> MEDVEIKPRGYQLRLVDHLTKSNGIVYLPTGSGKTFVAILVLKRFSQDFDKPIESGGKRALFMCNTVELARQQAMAVRRCTNFKVGFYVGEQGVDDWTRGMWSDEIKKNQVLVGTAQVFLDMVTQTYVALSSLSVVIIDECHHGTGHHPFREFMRLFTIANQTKLPRVVGLTGVLIKGNEITNVATKLKELEITYRGNIITVSDTKEMENVMLYATKPTEVMVSFPHQEQVLTVTRLISAEIEKFYVSLDLMNIGVQPIRRSKSLQCLRDPSKKSFVKQLFNDFLYQMKEYGIYAASIAIISLIVEFDIKRRQAETLSVKLMHRTALTLCEKIRHLLVQKLQDMTYDDDDDNVNTEEVIMNFSTPKVQRFLMSLKVSFADKDPKDICCLVFVERRYTCKCIYGLLLNYIQSTPELRNVLTPQFMVGRNNISPDFESVLERKWQKSAIQQFRDGNANLMICSSVLEEGIDVQACNHVFILDPVKTFNMYVQSKGRARTTEAKFVLFTADKEREKTIQQIYQYRKAHNDIAEYLKDRVLEKTEPELYEIKGHFQDDIDPFTNENGAVLLPNNALAILHRYCQTIPTDAFGFVIPWFHVLQEDERDRIFGVSAKGKHVISINMPVNCMLRDTIYSDPMDNVKTAKISAAFKACKVLYSLGELNERFVPKTLKERVASIADVHFEHWNKYGDSVTATVNKADKSKDRTYKTECPLEFYDALPRVGEICYAYEIFLEPQFESCEYTEHMYLNLQTPRNYAILLRNKLPRLAEMPLFSNQGKLHVRVANAPLEVIIQNSEQLELLHQFHGMVFRDILKIWHPFFVLDRRSKENSYLVVPLILGAGEQKCFDWELMTNFRRLPQSHGSNVQQREQQPAPRPEDFEGKIVTQWYANYDKPMLVTKVHRELTPLSYMEKNQQDKTYYEFTMSKYGNRIGDVVHKDKFMIEVRDLTEQLTFYVHNRGKFNAKSKAKMKVILIPELCFNFNFPGDLWLKLIFLPSILNRMYFLLHAEALRKRFNTYLNLHLLPFNGTDYMPRPLEIDYSLKRNVDPLGNVIPTEDIEEPKSLLEPMPTKSIEASVANLEITEFENPWQKYMEPVDLSRNLLSTYPVELDYYYHFSVGNVCEMNEMDFEDKEYWAKNQFHMPTGNIYGNRTPAKTNANVPALMPSKPTVRGKVKPLLILQKTVSKEHITPAEQGEFLAAITASSAADVFDMERLEILGNSFLKLSATLYLASKYSDWNEGTLTEVKSKLVSNRNLLFCLIDADIPKTLNTIQFTPRYTWLPPGISLPHNVLALWRENPEFAKIIGPHNLRDLALGDEESLVKGNCSDINYNRFVEGCRANGQSFYAGADFSSEVNFCVGLVTIPNKVIADTLEALLGVIVKNYGLQHAFKMLEYFKICRADIDKPLTQLLNLELGGKKMRANVNTTEIDGFLINHYYLEKNLGYTFKDRRYLLQALTHPSYPTNRITGSYQELEFIGNAILDFLISAYIFENNTKMNPGALTDLRSALVNNTTLACICVRHRLHFFILAENAKLSEIISKFVNFQESQGHRVTNYVRILLEEADVQPTPLDLDDELDMTELPHANKCISQEAEKGVPPKGEFNMSTNVDVPKALGDVLEALIAAVYLDCRDLQRT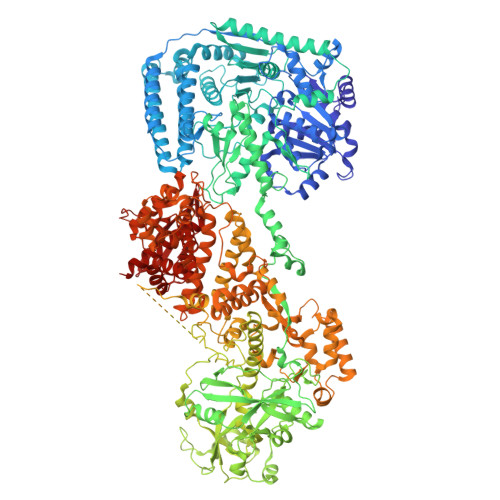WEVIFNLFEPELQEFTRKVPINHIRQLVEHKHAKPVFSSPIVEGETVMVSCQFTCMEKTIKVYGFGSNKDQAKLSAAKHALQQLSKCDA> PGREQQEENVPYLFKSQRFQSRFRASHGDFRILPKFTQRSQLLRGIEKFRVSVIELEPQSFMLPHHCDGEAIFVVVRGQGTISIAEQDEKNSFNLERGDVLRLHGGSTIHLLNRDNNEKFF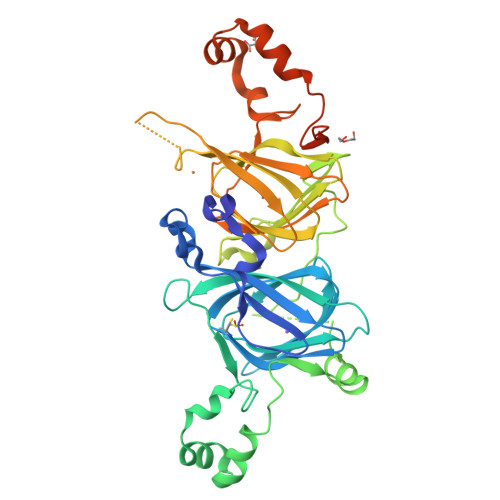VYVLAKSVNAPGQVQEYFSAGGENPESFYRAFSSDILESAFNTQRDRIERLFRQQKQGAIIKASEEQIRAISEHASRSTQQTRGRTQGPFNLMKERPQFGSRFGQFIEASPERFEQLRDLDAAVAFMNINQGGMVLPYYNSRSTRVVMVVEGNARFEMACPHLGRQGRGQGGEQEQEQEEGEVHYQKVRGNLNVGDVLVIPAGHPITFIATGGSNFRVVGFGINAMFNRKNFLAGRENIWRNIDREAKELSFNMPGREVEEIFQKQDQSYFVAGPEHRQQQPGERGEEGRKGQDQYLSSILDFVF>PPHLAALVLARGGSKGIPLKNIKRLAGVPLIGWVLRAALDAGVFQSVWVSTDHDEIENVAKQFGAQVHRRSSETSKDSSTSLDAIVEFLNYHNEVDIVGNIQATSPCLHPTDLQKVAEMIREEGYD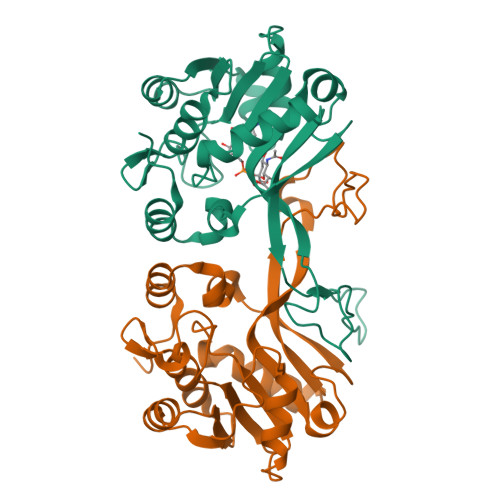SVFSVVRRHQFRWSEIQKGVREVTEPLNLNPAKRPRRQDWDGELYENGSFYFAKRHLIEMGYLQGGKMAYYEMRAEHSVDIDVDIDWPIAEQRVLRFGYFGKE[4x]Type IA topoisomerases (TopoIAs) are present in all living organisms. They resolve DNA/RNA catenanes, knots and supercoils by breaking and rejoining single-stranded DNA/RNA segments and allowing the passage of another nucleic acid segment through the break. Topoisomerase III-β (TOP3B), the only RNA topoisomerase in metazoans, promotes R-loop disassembly and translation of mRNAs. We present a series of cryo-EM structures of human TOP3B with its cofactor TDRD3 during cleavage and rejoining of DNA or RNA, thus elucidating the roles of divalent metal ions and key enzyme residues in each step of the catalytic cycle.

Yet, RNA complexes of TopoIA have not been previously visualized. We obtained RNA pre-cleavage and rejoining complexes of TOP3B. To obtain DNA- and RNA-bound TOP3B prior to cleavage, we substituted the nucleophile Y336, which forms tyrosyl-phosphate covalent bond with cleaved DNA, with a phenylalanine (F), to disable nucleic acid cleavage while preserving the DNA/RNA interactions. We prepared the cryo-EM sample by mixing cTOP3B-Y336F with DNA/RNA gap substrates in equimolar concentrations, and resolved the DNA and RNA complexes at an overall ~3.3 Å resolution revealing rigid components including protein and single-stranded nucleic acid fragments. As for ssDNA, TOP3B interacts with the ssRNA backbone through its charged amino-acid side chains, divalent-cation cofactors, and alpha-helix dipole moments. The backbone and base geometries of ssRNA and ssDNA are similar, with ssRNA establishing more backbone interactions. We observed that in the ssRNA bound to TOP3B structure, the upstream and downstream phosphate groups and bases are closer to the central scissile phosphate than those in ssDNA. Consequently, TOP3B exhibits a more compact structure with ssRNA than ssDNA, suggesting conformational flexibility upon binding to RNA or DNA. The catalytic sites of TOP3B are superimposable in the pre-cleavage DNA and RNA complexes, indicating a common mechanism employed by TOP3B for cleaving DNA and RNA.

> VMKTVLMVAEKPSLAQSIAKILSRGSLSSHKGLNGACSVHEYTGTFAGQPVRFKMTSVCGHVMTLDFLGKYNKWDKVDPAELFSQAPTEKKEANPKLNMVKFLQVEGRGCDYIVLWLDCDKEGENICFEVLDAVLPVMNKAHGGEKTVFRARFSSITDTDICNAMACLGEPDHNEALSVDARQELDLRIGCAFTRFQTKYFQGKYGDLDSSLISFGPCQTPTLGFCVERHDKIQSFKPETYWVLQAKVNTDKDRSLLLDWDRVRVFDREIAQMFLNMTKLEKEAQVEATSRKEKAKQRPLALNTVEMLRVASSSLGMGPQHAMQTAERLYTQGYISFPRTETTHYPENFDLKGSLRQQANHPYWADTVKRLLAEGINRPRKGHDAGDHPPITPMKSATEAELGGDAWRLYEYITRHFIATVSHDCKYLQSTISFRIGPELFTCSGKTVLSPGFTEVMPWQSVPLEESLPTCQRGDAFPVGEVKMLEKQTNPPDYLTEAELITLMEKHGIGTDASIPVHINNICQRNYVTVESGRRLKPTNLGIVLVHGYYKIDAELVLPTIRSAVEKQLNLIAQGKADYRQVLGHTLDVFKRKFHYFVDSIAGMDELMEVSF;> MAQVAGAALSQAGWYLSDEGIEACTSSPDKVNVNDIILIALNTDLRTIGKKFLPSDINSGKVEKLEGPCVLQIQKIRNVAAPKDNEESQAAPRMLRLQMTDGHISCTAVEFSYMSKISLNTPPGTKVKLSGIVDIKNGFLLLNDSNTTVLGGEVEHLIEKW>GPVDAPILLRQMFEPVSCTFTYLLGDRESREAVLIDPVLETAPRDAQLIKELGLRLLYAVNTHCHADHITGSGLLRSLLPGCQSVISRLSGAQADLHIEDGDSIRFGRFALETRASPGHTPGCVTFVLNDHSMAFTGDALLIRGCGRTDFQQGCAKTLYHSVHEKIFTLPGDCLIYPAHDYHGFTVSTVEEERTLNPRLTLSCEEFVKIMGNLNLPKPQQIDFAVPANMRCGVQTPTA[2x]

EE is caused by mutations to the gene (HGNC: 23287) encoding for the ethylmalonic encephalopathy protein 1 (ETHE1, also known as sulphur dioxygenase, SDO) and correlates with increased cellular levels of hydrogen sulfide. ETHE1 is a non-heme iron-dependent oxygenase that catalyses the biochemically interesting oxidation of glutathione persulfide (GSSH) to give glutathione and persulfite [Eq. (1)]. ETHE1 is reported to be localized to mitochondria where its activity is linked to electron transfer chain energy generation and is of central importance in hydrogen sulfide metabolism. Sequence analyses predict that hETHE1 is a member of the widely distributed metallo-β-lactamase (MBL)-fold family.

Recombinant hETHE1 lacking its 20 residue N-terminal mitochondrial targeting sequence was produced in Escherichia coli and highly purified (≥95%) as determined by sodium dodecyl sulfate-polyacrylamide gel electrophoresis (SDS-PAGE) analysis. hETHE1 was crystallized using the sitting drop vapour diffusion method. The final model (orthorhombic space group P212121) has two chains representing the dimer in the asymmetric unit. The hETHE1 structure reveals an αββα MBL-type fold with two central mixed β-sheets, each containing six strands, surrounded on both sides by helices. Non-denaturing mass spectrometric and multi-angle laser light scattering (MALS) analyses indicate that hETHE1 is predominantly dimeric with some monomer also being observed (dimer to monomer ratio ∼10:1); quantitative gel filtration analysis indicated a mass for hETHE1 intermediate between monomeric (26 116 Da) and dimeric (52 232 Da) forms in solution. The total buried surface area at the interface is 1950 Å2 and the calculated free energy of binding (ΔG) for the dimer is about −37 kcal/mol. The active site of each hETHE1 protomer in the asymmetric unit contains a single iron ion. Interestingly, three of five characteristic MBL family metal-binding motif residues, His79, His135 and Asp154 (corresponding to His118, His196, and Cys221, BBL numbering system), act as iron coordinating residues in hETHE1. Three water molecules complete the metal coordination. Residues His81ETHE1 (His118BBL), Asp83ETHE1 (Asp120BBL) and His195ETHE1 (His263BBL) are present in the hETHE1 active site, but are not involved in metal coordination as observed in the current structural data. Analysis of the enzyme surface reveals a channel, comprised of residues 163–166 and 226–232, leading to the active site that is sufficient to accommodate a substrate molecule of GSSH; this channel is apparently conserved in the A. thaliana ETHE1.>MAIERTLSIVKPDAVSKNHIGEIFARFEKAGLKIVATKMKHLSQADAEGFYAEHKERGFFGDLVAFMTSGPVVVSVLEGENAVLAHREILGATNPKEAAPGTIRADFAVSIDENAAHGSDSVASAERE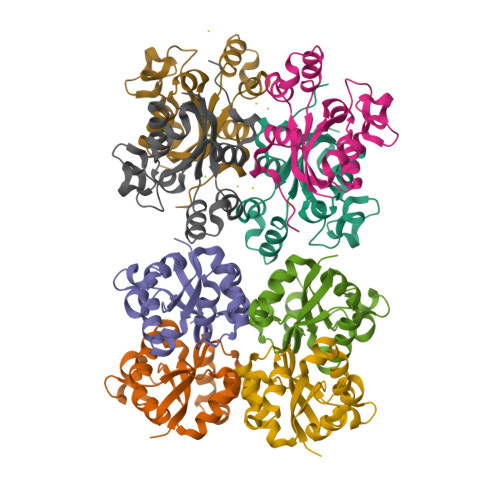IAYFFADNEICPRTR[8x]>[4x]MPLYVIDKPITLHILTQLRDKYTDQINFRKNLVRLGRILGYEISNTLDYEIVEVETPLGVKTKGVDITDLNNIVIINILRAAVPL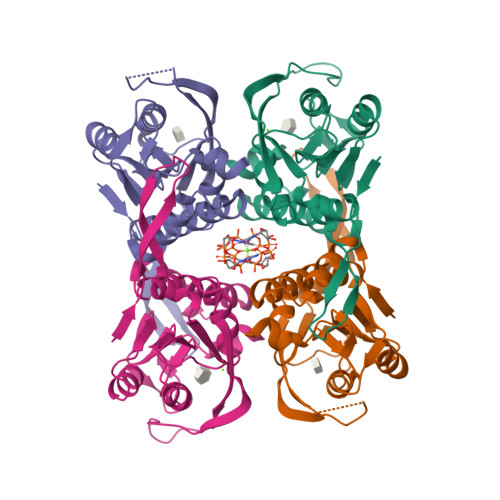VEGLLKAFPKARQGVIGASRVEVDGKEVPKDMDVYIYYKKIPDIRAKVDNVIIADPMIATASTMLKVLEEVVKANPKRIYIVSIISSEYGVNKILSKYPFIYLFTVAIDPELNNKGYILPGLGDAGDRAFG>[6x]MASWSHPQFEKIEGREPLHLPILEFKTEYRYPSTFEHEAQFKDTVLEFLAHEASDIIIKQGVAISAKVKGTLCTLSTRTLNFNEIERIALWASGSSSVLTELASKKLINTRYEVFHPTKLTTGGQKQRFGYRVNISPVYIQGKTTAEIVMRSIPLDPLPLADIGLSPELVNQMCPDNGIVMVAGKTSSGKSTTFSSIIRYIMENDTPIKGHLLTHEDPIEFVYDNIKSAHSIIAQSQIPE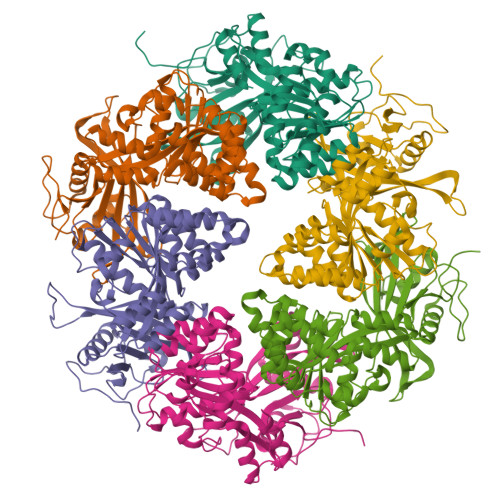QFSSFAIANQEALRRTPNLIMIGELRDKQSIESAFEAANTGHPVFATVHSQNCSAVMRRLISRFDESVRGAAIYDLVETTRFIMAQTLVRKTDGNLVAAREYLNFTTDIREQLLSLSDMGKVASEVRRLVDEFGHPFSLEAERLHSDGIIDGHVAKRLSMMS> KRPPKLGQIGRS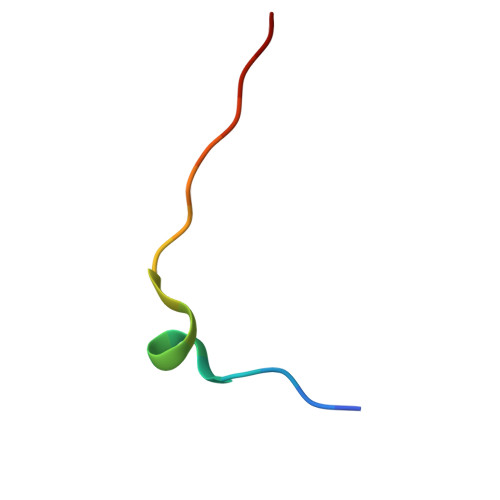KRVVIA> NNINKTRMNDLNREETRLKTFTDWPLDWLDKRQLAQTGMYFTHAGDKVKCFFCGVEIGSWEQEDQPVPEHQRWSPNCPLLRRRTTNNVPINAEALDRILPPISYDICGAND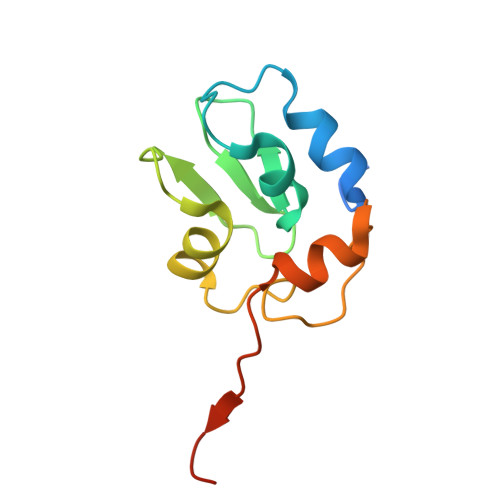STLE>MDSLDQCIVNACKNSWDKSYLAGTPNKDNCSGFVQSVAAELGVPMPRGNANAMVDGLEQSWTKLASGAEAAQKAAQGFLVIAGLKGRTYGHVAVVISGPLYRQKYPMCWCGSIAGAVGQSQGL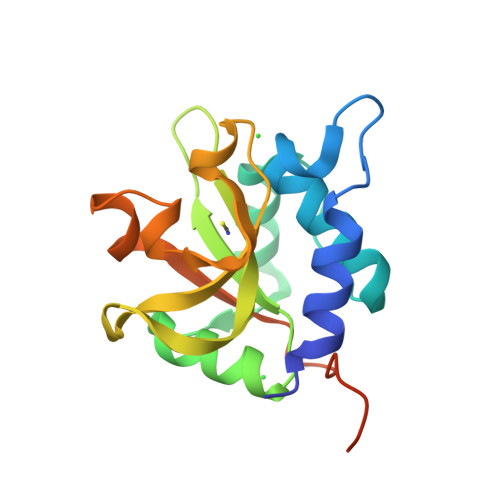KSVGQVWNRTDRDRLNYYVYSLASCSLPRASAAALEHHHHHH[4x]>GSKTISESELSASATELLQDYMLTLRTKLSSQEIQQFAALLHEYRNGASIHEFCINLRQLYGDSRKFLLLGL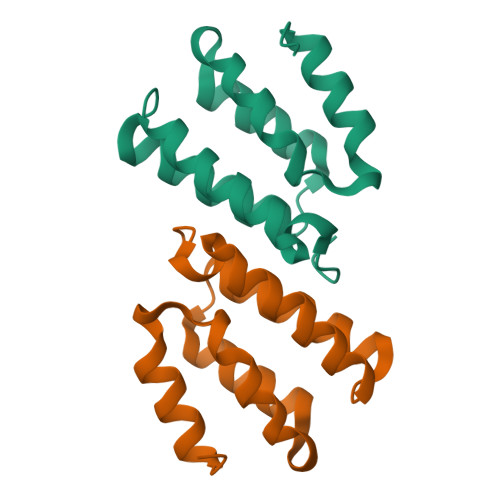RPFIPEKDSQHFENFLETIGVKDGRG[4x]>RKKGGWFGKHRGQGGSNPKFENIAEGLRVLLARSHVERTTEEGNWVAGVFVYGGSKTSLYNLRRGIALAVPQCR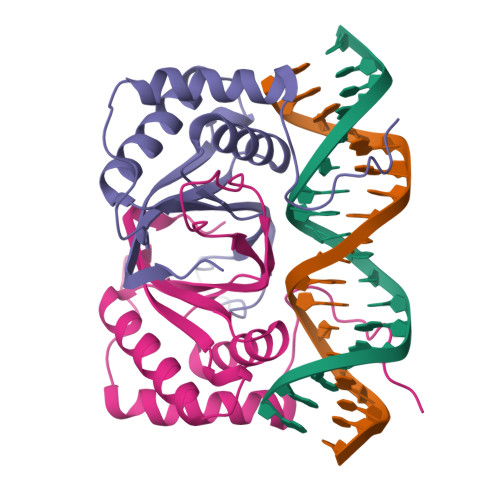ITPLSRLPFGMAPGPGPQPGPLRESIVCYFMVFLQTHIFAEVLKDAIKDLVMIKPAPTCNIKVTVCSFDDGVDLP[2x]>MGRGKVKPNRKSTGDNSNVVTMIRAGSYPKVNPTPTWVRAIPFEVSVQSGIAFKVPVGSLFSANFRTDSFTSVTVMSVRAWTQLTPPVNEYSFVRLKPLFKTGDSTEEFEGRASNINTRASVGYRIPTNLRQNTVAADNVCEVRSNCRQVALVISCC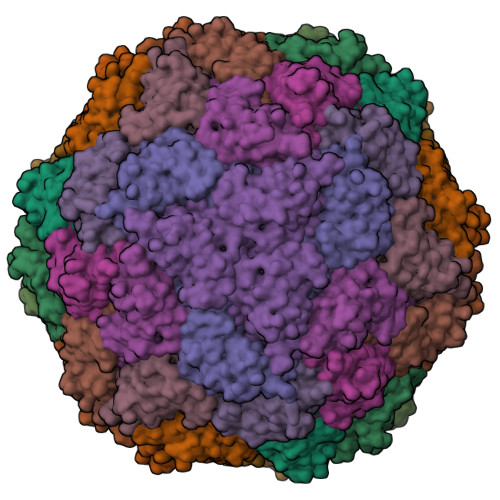FN[20x]>MSEFNITETYLRFLEEDTEMTMPIAAIEALVTLLRIKTPETAAEMINTIKSSTEELIKSIPNSVSLRAGCDIFMRFVLRNLHLYGDWENCKQHLIENGQLFVSRAKKSRNKIAEIGVDFIADDDIILVHGYSRAVFSLLNHAANKFIRFRCVVTESRPSKQGNQLYTLLEQKGIPVTLIVDSAVGAVIDKVDKVFVGAEGVAESGGIINLVGTYSVGVLAHNARKPFYVVTESHKFVRMFPLSSDDLPMAGPPLDFTRRTDDLEDALRGPTIDYTAQEYITALITDLGVLTPSAVSEELIKMWYD[2x];>[2x]MSSQAFTSVHPNAATSDVNVTIDTFVAKLKRRQVQGSYAIALETLQLLMRFISAARWNHVNDLIEQIRDLGNSLEKAHPTAFSCGNVIRRILAVLRDEVEEDTMSTTVTSTSVAEPLISSMFNLLQKPEQPHQNRKNSSGSSSMKTKTDYRQVAIQGIKDLIDEIKNIDEGIQQIAIDLIHDHEILLTPTPDSKTVLKFLITARERSNRTFTVLVTEGFPNNTKNAHEFAKKLAQHNIETLVVPDSAVFALMSRVGKVIIGTKAVFVNGGTISSNSGVSSVCECAREFRTPVFAVAGLYKLSPLYPFDVEKFVEFGGSQRILPRMDPRKRLDTVNQITDYVPPENIDIYITNVGGFNPSFIYRIAWDNYKQIDVHLDKNKA;>MSIQAFVFCGKGSNLAPFTQPDFPFQTQNKDSTAATSGDKLNELVNSALDSTVINEFMQHSTRLPKALLPIGNRPMIEYVLDWCDQADFKEISVVAPVDEIELIESGLTSFLSLRKQQFELIYKALSNSNHSHHLQDPKKINFIPSKANSTGESLQKELLPRINGDFVILPCDFVTDIPPQVLVDQFRNRDDNNLAMTIYYKNSLDSSIDKKQQQKQKQQQFFTVYSENEDSERQPILLDVYSQRDVTKTKYLQIRSHLLWNYPNLTVSTKLLNSFIYFCSFELCQLLKLGPQSMSRQASFKDPFTGNQQQQNPPTTDDDEDRNHDDDDDYKPSATSIQPTYFKKKNDLILDPINCNKSLSKVFRDLSRRSWQHSKPREPIGIFILPNETLFIRANNLNAYMDANRFVLKIKSQTMFTKNIQIQSAAIGADAIVDPKCQISAHSNVKMSVLGTQANIGSRCRVAGSLLFPGVHLGDEVILENCIIGPMAKIGSKCKLSNCYIEGHYVVEPKNNFKGETLANVYLDEDEEDELIYDDSVIAGESEIAEETDSDDRSDEDSDDSEYTDEYEYEDDGLFER[2x];>[2x]MSESEAKSRSATPPSKAKQATPTTTAAANGEKKLTNKELKELKKQEKAAKRAAMKQANGISIEQQQQQAQMKKEKKQLQREQQQKREQKQKNANKKKQNERNVKKSTLFGHLETTEERRATILALTSAVSSPKTSRITAAGLMVPVVASALSGSNVLTASSLMPVGPNASSTVSASAPASTTTTLPASSAALSAGTSSASTNTPTAIQQEIASSNASDVAKTLASISLEAGEFNVIPGISSVIPTVLEQSFDNSSLISSVKELLLNKDLIHPSILLLTSHLAHYKIVGSIPRCIAMLEVFQIVIKDYQTPKGTTLSRNLTSYLSHQIDLLKKARPLSVTMGNAIRWLKQEISLIDPSTPDKAAKKDLCEKIGQFAKEKIELADQLIIDNASTQIEESTTIVTYGSSKVLTELLLHNAISLKKNIKVIVVDSRPLFEGRKMAETLRNAGVNVMYALITSLDTIFNMDVDYVFLGAHSILSNGFLYSRAGTAMLAMSAKRRNIPVLVCCESLKFSQRVQLDSVTFNELADPNDLVNIDYENPVERRGNKGALLNQFIKERKFEKKKLAMENKPKGNKIGGKKGSEGESKDASNEEDSNSKNILDGWQELPSLNIVNILYDLTPPEYIKKVITEFGALPPSSVPVILREYKGSA;>MAGKKGQKKSGLGNHGKNSDMDVEDRLQAVVLTDSYETRFMPLTAVKPRCLLPLANVPLIEYTLEFLAKAGVHEVFLICSSHANQINDYIENSKWNLPWSPFKITTIMSPEARCTGDVMRDLDNRGIITGDFILVSGDVLTNIDFSKMLEFHKKMHLQDKDHISTMCLSKASTYPKTRTIEPAAFVLDKSTSRCIYYQDLPLPSSREKTSIQIDPELLDNVDEFVIRNDLIDCRIDICTSHVPLIFQENFDYQSLRTDFVKGVISSDILGKHIYAYLTDEYAVRVESWQTYDTISQDFLGRWCYPLVLDSNIQDDQTYSYESRHIYKEKDVVLAQSCKIGKCTAIGSGTKIGEGTKIENSVIGRNCQIGENIRIKNSFIWDDCIIGNNSIIDHSLIASNATLGSNVRLNDGCIIGFNVKIDDNMDLDRNTKISASPLKNAGSRMYDNESNEQFDQDLDDQTLAVSIVGDKGVGYIYESEVSDDEDSSTEACKE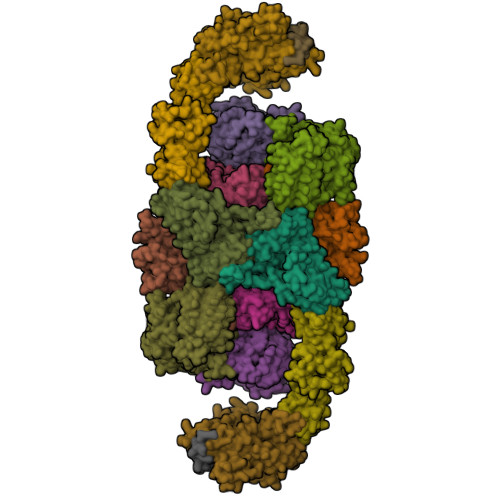INTLSNQLDELYLSDDSISSATKKTKKRRTMSVNSIYTDREEIDSEFEDEDFEKEGIATVERAMENNHDLDTALLELNTLRMSMNVTYHEVRIATITALLRRVYHFIATQTLGPKDAVVKVFNQWGLLFKRQAFDEEEYIDLMNIIMEKIVEQSFDKPDLILFSALVSLYDNDIIEEDVIYKWWDNVSTDPRYDEVKKLTVKWVEWLQNADEESSSEEE[2x];>[2x]MSTSHCRFYENKYPEIDDIVMVNVQQIAEMGAYVKLLEYDNIEGMILLSELSRRRIRSIQKLIRVGKNDVAVVLRVDKEKGYIDLSKRRVSSEDIIKCEEKYQKSKTVHSILRYCAEKFQIPLEELYKTIAWPLSRKFGHAYEAFKLSIIDETVWEGIEPPSKDVLDELKNYISKRLTPQAVKIRADVEVSCFSYEGIDAIKDALKSAEDMSTEQMQVKVKLVAAPLYVLTTQALDKQKGIEQLESAIEKITEVITKYGGVCNITMPPKAVTATEDAELQALLESKELDNRSDSEDDEDESDDE;>MSDLQDQEPSIIINGNLEPVGEPDIVEETEVVAQETQETQDADKPKKKVAFTGLEEDGETEEEKRKREFEEGGGLPEQPLNPDFSKLNPLSAEIINRQATINIGTIGHVAHGKSTVVRAISGVQTVRFKDELERNITIKLGYANAKIYKCQEPTCPEPDCYRSFKSDKEISPKCQRPGCPGRYKLVRHVSFVDCPGHDILMSTMLSGAAVMDAALLLIAGNESCPQPQTSEHLAAIEIMKLKHVIILQNKVDLMREESALEHQKSILKFIRGTIADGAPIVPISAQLKYNIDAVNEFIVKTIPVPPRDFMISPRLIVIRSFDVNKPGAEIEDLKGGVAGGSILNGVFKLGDEIEIRPGIVTKDDKGKIQCKPIFSNIVSLFAEQNDLKFAVPGGLIGVGTKVDPTLCRADRLVGQVVGAKGHLPNIYTDIEINYFLLRRLLGVKTDGQKQAKVRKLEPNEVLMVNIGSTATGARVVAVKADMARLQLTSPACTEINEKIALSRRIEKHWRLIGWATIKKGTTLEPIA[2x];>MSSDLAAELGFDPALKKKKKTKKVIPDDFDAAVNGKENGSGDDLFAGLKKKKKKSKSVSADAEAEKEPTDDIAEALGELSLKKKKKKTKDSSVDAFEKELAKAGLDNVDAESKEGTPSANSSIQQEVGLPYSELLSRFFNILRTNNPELAGDRSGPKFRIPPPVCLRDGKKTIFSNIQDIAEKLHRSPEHLIQYLFAELGTSGSVDGQKRLVIKGKFQSKQMENVLRRYILEYVTCKTCKSINTELKREQSNRLFFMVCKSCGSTRSVSSIKTGFQATVGKRRRM[2x]> MAGDPNSMTVSHHNASTARFYALRLLPGQEVFSQLHAFVQ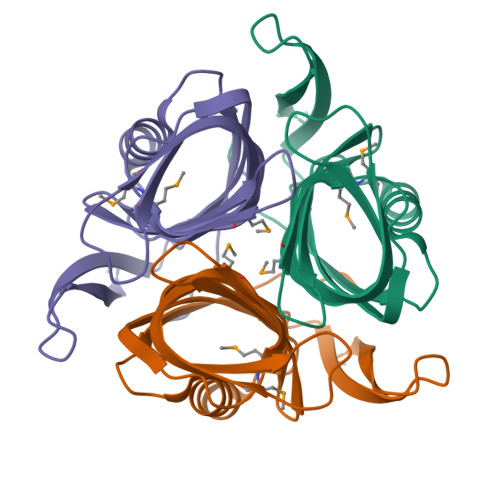QNQLRAAWIAGCTGSLTDVALRYAGQEATTSLTGTFEVISLNGTLELTGEHLHLAVSDPYGVMLGGHMMPGCTVRTTLELVIGELPALTFSRQPCAISGYDELHISSRLEHHHHHH> MTTAAGLSGIDLTDLDNFADGFPHHLFAIHRREAPVYWHRPTEHTPDGEGFWSVATYAETLEVLRDPVTYSSVTGGQRRFGGTVLQDLPVAGQVLNMMDDPRHTRIRRLVSSGLTPRMIRRVEDDLRRRARGLLDGVEPGAPFDFVVEIAAELPMQMICILLGVPETDRHWLFEAVEPGFDFRGSRRATMPRLNVEDAGSRLYTYALELIAGKRAEPADDMLSVVANATIDDPDAPALSDAELYLFFHLLFSAGAETTRNSIAGGLLALAENPDQLQTLRSDFELLPTAIEEIVRWTSPSPSKRRTASRAVSLGGQPIEAGQKVVVWEGSANRDPSVFDRADEFDITRKPNPHLGFGQGVHYCLGANLARLELRVLFEELLSRFGSVRVVEPAEWTRSNRHTGIRHLVVELRGG

Among these is CYP126A1, a P450 with ∼35% amino acid identity to the cholesterol-oxidizing M. tuberculosis CYP142A1 and CYP125A1. However, CYP126A1 is highly conserved across pathogenic and non-pathogenic Mycobacterium species, suggesting an important evolutionary role for the protein. In conclusion, we present the first biochemical and structural studies of the M. tuberculosis P450 CYP126A1, revealing novel substrates and inhibitors for the enzyme, defining its relatively polar active site and its ability to adapt structurally to facilitate the binding of bulky ligands. The CYP126A1 structures reveal a dynamic molecule, with the BC and FG regions clearly affected by ligand binding.

The CYP126A1 Kd for ketoconazole is 0.34 ± 0.07 μm, whereas imidazole binds substantially more weakly (Kd = 2.59 ± 0.06 mm). For example, ketoconazole induces a Soret shift from 418.5 to 423.5 nm at apparent saturation, in addition to inducing smaller absorbance changes in the heme α- and β-band peaks (minor shifts to ∼569.5 and 540.5 nm, respectively, with notably decreased intensity of the α-band). However, ketoconazole binds in a different manner and extends from the heme in an orthogonal direction to the other two molecules. The distinctive binding mode for ketoconazole has ramifications for the structural organization of CYP126A1. The crystal structure of CYP126A1 in complex with the azole drug ketoconazole revealed that a large scale reorientation of the BC-loop region has occurred in response to ligand binding, disrupting the putative dimer interface observed in the imidazole-bound form. Furthermore, the N-terminal region of the I-helix and the associated FG-helices display comparatively more modest reorientations as a consequence of ligand binding. The ketoconazole dichlorobenzene moiety occupies the region previously filled by Leu-249, whereas the extended tail of the molecule displaces the BC-loop residues Val-84 and Leu-85, resulting in their forming hydrophobic contacts with the FG-helices. In contrast, the CYP126A1-ketoconazole structure is a crystallographic monomer. Ketoconazole binding reorients the BC-loop region of CYP126A1 and disrupts the dimer interface, resulting in a binding mode for ketoconazole that is approximately orthogonal to those for HTS compounds 1 and 7, which extend upward from the heme, close to the path followed by the I-helix. The formation of ligand-protein complexes at substoichiometric ligand/protein ratios for ketoconazole and compounds 1, 3, and 7 indicates strong gas phase binding.>GIGTGFPFDPHYVEVLGERMHYVDVGPRDGTPVLFLHGNPTSSYVWRNIIPHVAPTHRCIAPDLIGMGKSDKPDLGYFFDDHVRFMDAFIEALGLEEVVLVIHDWGSALGFHWAKRNPERVKGIAFMEFIRPIPTWDEWPEFARETFQAFRTTDVGRKLIIDQNVFIEGTLPMGVVRPLTEVEMDHYREPFLNPVDREPLWRF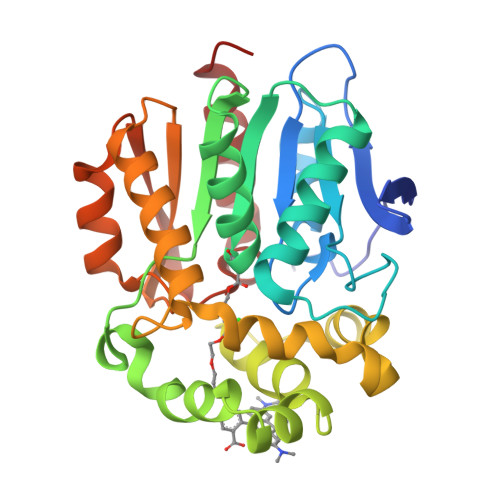PNELPIAGEPANIVALVEEYMDWLHQSPVPKLLFWGTPGVLIPPAEAARLAKSLPNCKAVDIGPGLNLLQEDNPDLIGSEIARWLSTLEI[5x]>MTPHINAKIGDFYPQCLLCGDPLRVSYIAKKFLQDAKEITNVRNMLGFSGKYKGRGISLMGHGMGIASCTIYVTELIKTYQVKELLRIGTCGAISPKVGLKDIIMATGASTDSKTNRVRFLNHDLSATPDFELSLRAYQTAKRLGIDLKVGNVFSSDFFYSFETHAFDLMAKYNHLAIEMEAAGLYATAMEL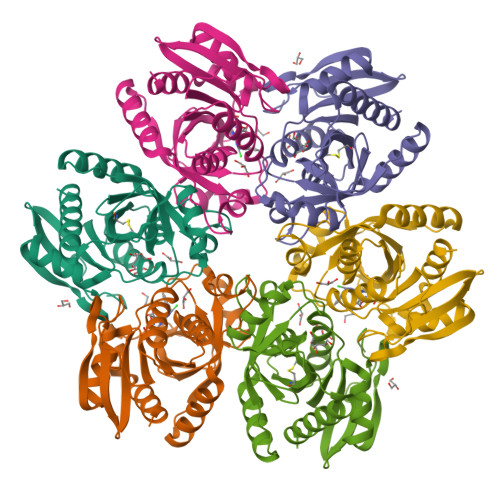NAKALCLCSVSDHLITKEALSPKERVESFDNMIILALEMMS[2x]>[4x]GSHMSAPLPLDELRTFAEVLDRVKAAYVEPVDDKTLLENAIKGMLSNLDPHSAYLGPEDFAELQESTSGEFGGLGIEVGSEDGFIKVVSPIDDTPAARAGIQPGDLIVQIDGKPTKGQSMTEAVDSMRGKAGSPITLTIVRDGGRPFDVELKRAIIKVKSVKSQVLEPGYAYLRITQFQVNTGEEVVKALNQLRKDNKGRLKGLVLDLRNNPGGVLQSAVEVADAFLTKGLIVYTKGRIANSELRFSADPADPSDKVPLVVLINGGSAAAAEIVAGALQDQKRAILMGTDSFGKGSVQTVLPLNNDRALKLTTALYYTPNGRSIQAQGIVPDIEVGRAKVTQERSSFEGFKEADLQGHLANGNGGADRPTGKRAAPSERPQDSDYQLSQALSLLKGLSVTRGN;> MEDTAVETKAKPEKYGSFSEDSLYSLLVAELAGQRNRFDIALSNYVVQAQKTRDPGVSERAFRIAEYLGADQEALDTSLLWARSAPDNLDAQRAAAIQLARAGRYEESMVYMEKVLNGQGDTHFDFLALSAAETDPDTRAGLLQSFDHLLKKYPNNGQLLFGKALLLQQDGRPDEALTLLEDNSASRHEVAPLLLRSRLLQSMKRSDEALPLLKAGIKEHPDDKRVRLAYARLLVEQNRLDDAKAEFAGLVQQFPDDDDLRFSLALVCLEAQAWDEARIYLEELVERDSHVDAAHFNLGRLAEEQKDTARALDEYAQVGPGNDFLPAQLRQTDVLLKAGRVDEAAQRLDKARSEQPDYAIQLYLIEAEALSNNDQQEKAWQAIQEGLKQYPEDLNLLYTRSMLAEKRNDLAQMEKDLRFVIAREPDNAMALNALGYTLADRTTRYGEARELILKAHKLNPDDPAILDSMGWINYRQGKLADAERYLRQALQRYPDHEVAAHLGEVLWAQGRQGDARAIWREYLDKQPDSDVLRRTIKRLTGAETP

During bacterial cell growth, hydrolases cleave peptide cross-links between strands of the peptidoglycan sacculus to allow new strand insertion. The Pseudomonas aeruginosa carboxyl-terminal processing protease (CTP) CtpA regulates some of these hydrolases by degrading them. CtpA assembles as an inactive hexamer composed of a trimer-of-dimers, but its lipoprotein binding partner LbcA activates CtpA by an unknown mechanism. LbcA has an N-terminal adaptor domain that binds to CtpA, and a C-terminal superhelical tetratricopeptide repeat domain.

We next carried out a local refinement focusing on the upper one-third region of the complex containing a CtpA dimer and the best LbcA density, which obtained an EM map at an average resolution of 3.55 Å. The structure comprises two CtpA monomers, a substrate peptide, and the N-terminal region of LbcA. In the atomic model LbcA approaches the CtpA dimer from the front and is ordered in the N-terminal adaptor domain. Interestingly, only the front CtpA is in an activated configuration while the back CtpA remains inactive. We found that the LbcA N-terminal α-helix 1 (H1) inserts into a space between the two H1 of the CtpA dimer. The space between the two CtpA H1 is widened by 8 Å to accommodate the LbcA H1. The CtpA–LbcA interface is dominated by hydrophobic interactions. However, in the front CtpA, all distances between Ala-302, Lys-327, and Gln-331 are shortened to below 3.3 Å, except for the distance between Ala-302 and Lys-327 that is shortened to only 5.2 Å. In addition, the cap has lowered down by 8 Å to narrow down the substrate pocket to 8.7 Å, perhaps leading to the trapping of an endogenous substrate peptide in the narrowed substrate binding pocket. We tentatively assigned this density as a substrate peptide that co-purified with the protease and have built a seven-alanine atomic model in the linear density.>[4x]SHSEEPAEILPPARDEEEEEEEGMEQGLEEEEEVDPRIQGELEKLNQSTDDINRRETELEDARQKFRSVLVEATVKLDELVKKIGKAVEDSKPYWEARRVARQAQLEAQKATQDFQRATEVLRAAKETISLAE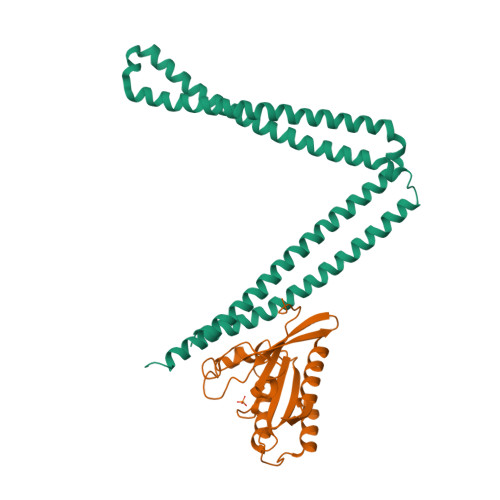QRLLEDDKRQFDSAWQEMLNHATQRVMEAEQTKTRSELVHKETAARYNAAMGRMRQLEKKLKRAINKSKPYFELKAKYYVQLEQLKKTVDDLQAKLTLAKGEYKMALKNLEMISDEIHERRRSSAMGPRGCGVGAE;>SHMGTRDDEYDYLFKVVLIGDSGVGKSNLLSRFTRNEFNLESKSTIGVEFATRSIQVDGKTIKAQIWDTAGQERYRAITSAYYRGAVGALLVYDIAKHLTYENVERWLKELRDHADSNIVIMLVGNKSDLRHLRAVPTDEARAFAEKNGLSFIETSALDSTNVEAAFQTILTEIY[4x]>PSVYDAAAQLTADVKKDLRDSWKVIGSDKKGNGVALMTTLFADNQETIGYFKRLGDVSQGMANDKLRGHSITLMYALQNFIDQLDNPDDLVCVVEK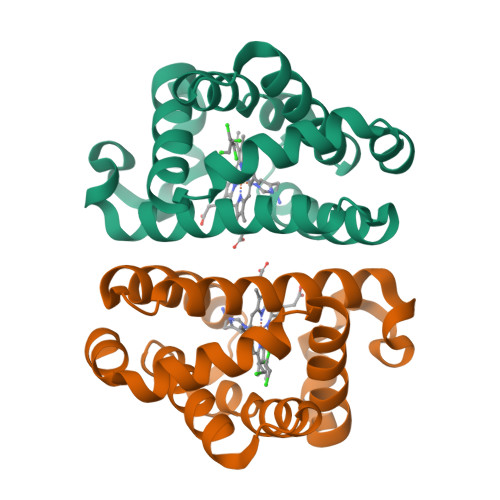FAVNHITRKISAAEFGKINGPIKKVLASKNFGDKYANAWAKLVAVVQAAL[2x]>SNAMDFHIRKATNSDAEAIQHVATTSWHHTYQDLIPSDVQDDFLKRFYNVETLHNRISATPFAVLEQADKVIGFANFIELEKGKSELAAFYLLPEVTQRGLGTELLEVGMTLFHVPLPMFVNVEKGNETAIHFYKAKGFVQVEEFTEDFYGYPL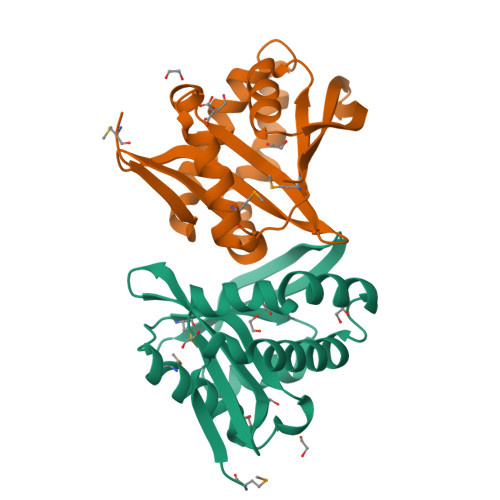ETIRFNLNH[2x]6-bromanyl-1~{H}-indazol-4-amine | C7 H6 Br N3 | 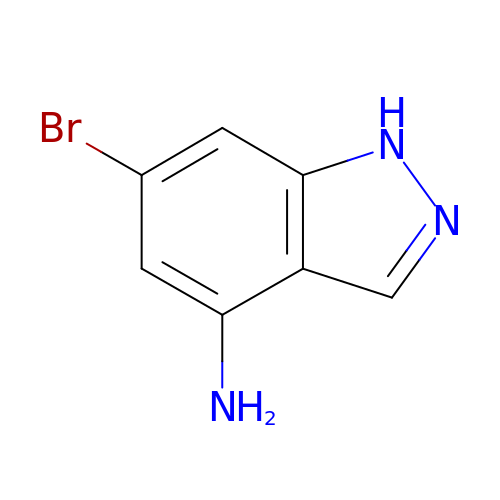JORDVWJEXMDSBI-UHFFFAOYSA-N> IVGGEDAKPGQFPWQVVLNGKVDAFCGGSIVNEKWIVTAAHCVETGVKITVVAGEHNIEETEHTEQKRNVIRIIPHHNYNAAINTYNHDIALLELDEPLVLNSYVTPICIADKEYTNIFLKF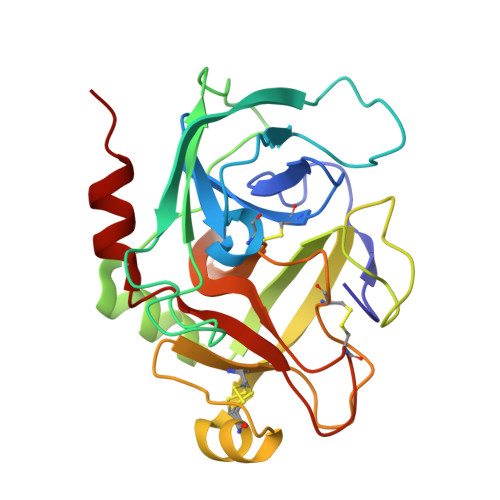GSGYVSGWGRVFHKGRSALVLQYLRVPLVDRATCLRSTKFTITNNMFCAGFHEGGRDSCQGDSGGPHVTEVEGTSFLTGIVSWGEECAMKGKYGIYTKVSRYVNWIKEKTKLT> FEARLVQGSILKKVLEALKDLINEACWDISSSGVNLQSMDSSHVSLVQLTLRSEGFDTYRCDRNLAMGVNLTSMSKILKCAGNEDIITLRAEDNADTLALVFEAPNQEKVSDYEMKLMDLDVEQLGIPEQEYSCVVKMPSGEFARICRDLSHIGDAVVISCAKDGVKFSASGELGNGNIKLSQTSNVDKEEEAVTIEMNEPVQLTFALRYLNFFTKATPLSSTVTLSMSAD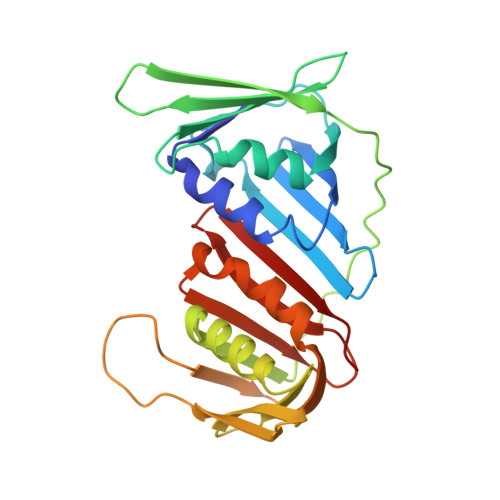VPLVVEYKIADMGHLKYYLAPK> MGSSHHHHHHSSGLVPRGSHPSLRTQPSLYSGPFPFYRRPSELGCFSLDAQRQYHGDARALRYYSPPPINGPGPDFDLRDGYPDRYQPRDEEVQERLDHLLRWVLEHRNQLEGGPGWLAGATVTWRGHLTKLLTTPYERQEGWQLAASRFQGTLYLSEVETPAARAQRLARPPLLRELMYMGYKFEQYM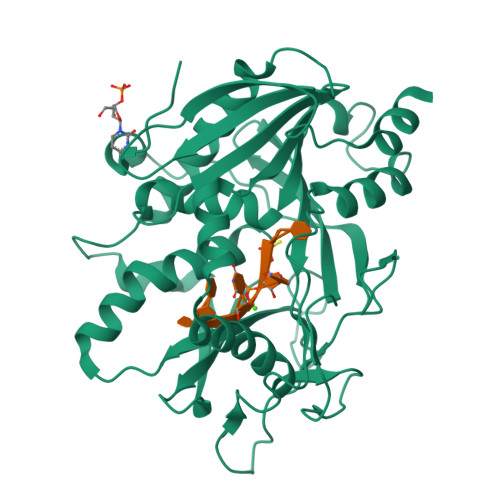CADKPGGSPDPSGEVNTNVAYCSVLRSRLGNHPLLFSGEVDCLNPQAPCTQPPSCYVELKTSKEMHSPGQWRSFYRHKLLKWWAQSFLPGVPHVVAGFRNPEGFVCSLKTFPTMEMFENVRNDREGWNPSVCMNFCAAFLSFAQSTVVQDDPRLVHLFSWEPGGPVTVSVHRDAPYAFLPSWYVETMTQ>[2x]MRGSHHHHHHGSPIKVGDIIPDVLVYEDVPSKSFPIHDVFRGRKGILF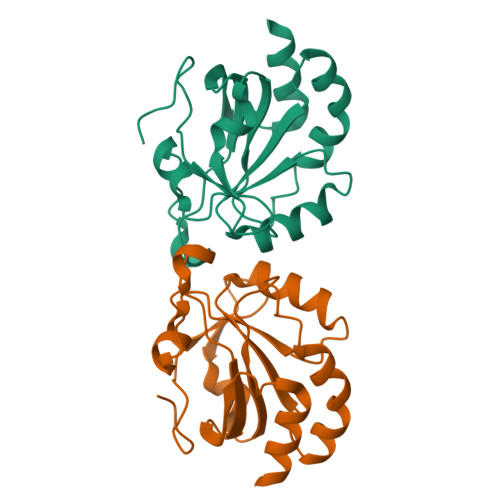SVVGAFVPGSNNHIPEYLSLYDKFKEEGYHTIACIAVNDPFVMAAWGKTVDPEHKIRMLADMHGEFTRALGTELDSSKMLGNNRSRRYAMLIDDNKIRSVSTEPDITGLACLLSIQRQKENKT> MKRVITLFAVLLMGWSVNAWSFACKTANGTAIPIGGGSANVYVNLAPVVNVGQNLVVDLSTQIFCHNDYPETITDYVTLQRGSAYGGVLSNFSGTVKYSGSSYPFPTTSETPRVVYNSRTDKPWPVALYLTPVSSAGGVAIKAGSLIAVLILRQTNNYNSDDFQFVWNIYANNDVVVPTGGCDVSARDVTVTLPDYPGSVPIPLTVYCAKSQNLGYYLSGTTADAGNSIF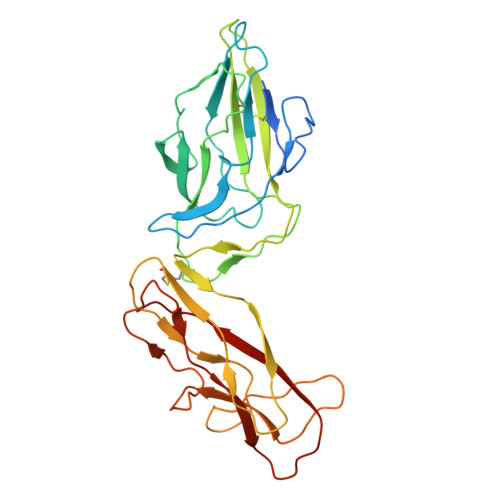TNTASFSPAQGVGVQLTRNGTIIPANNTVSLGAVGTSAVSLGLTANYARTGGQVTAGNVQSIIGVTFVYQ[(5S)-5-amino-5-carboxyhexyl](trihydroxy)borate | C7 H17 B N O5 | 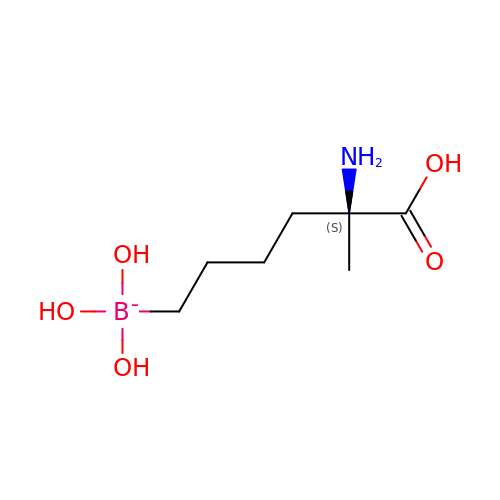QCQHNLBDTJIODE-ZETCQYMHSA-N> MSTNSFDGSIVSSYLTTRMPPWAGVRQNVMGSSIDGRPVLPANSTTLTYETVSGTPLETAASAAASAAAATARGIVTDFAFLSPLASSAASRSSARDDKLTALLAQLDSLTRELNVVSQQLLDLRQQVSA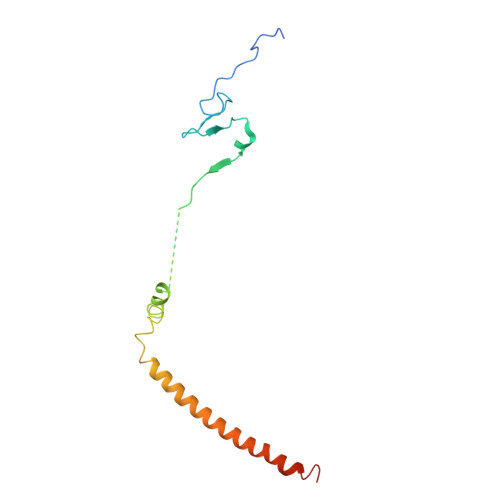LKASSPPNAV>[2x]AITGIFFGSDTGNTENIAKMIQKQLGKDVADVHDIAKSSKEDLEAYDILLLGIP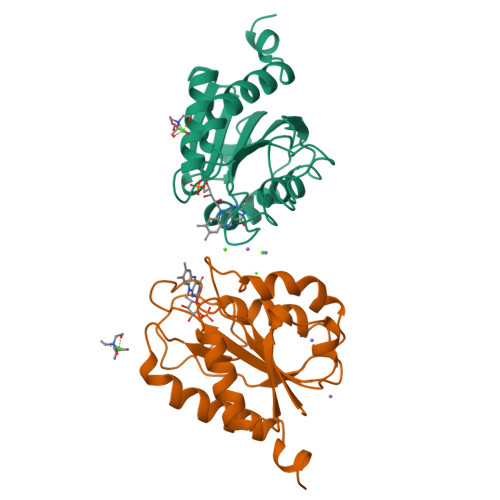TWYYGEAQCDWDDFFPTLEEIDFNGKLVALFGCGDQEDYAEYFCDALGTIRDIIEPRGATIVGHWPTAGYHFEASKGLADDDHFVGLAIDEDRQPELTAERVEKWVKQISEELHLDEILNA>GPLGSETKENRWVPVTVLPGCVGCRTVAALASWTVRDVKERIFAETGFPVSEQRLWRGGRELSDWIKIGDLTSKNCHLFVNMQSKGLKG[2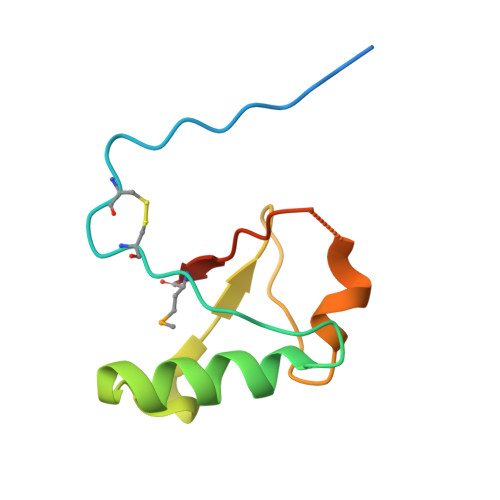x]> MKKLILLTLIIASFDIYAIDFVYRVDPNPPDVIFR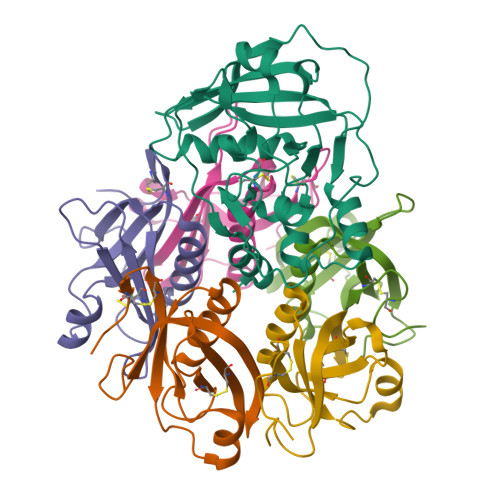DGFSLLGYNRDLQQLISGRSCAGGSSDSRYIVTTSDINKTYAIARAYYSHSKFKGNLYRYKIRADNNFYSLTPSVNYLESQGGHFNAYEKSMIRLQSEYVSTLSILPENIQKAVALVYDSSTGQIKDGTSTINTDYVSISSVSNPGVIPFLPEPQANTQQRIDAFGSLISSCFSIYSVCQTHRGQKTEVYKMPFYDARPVIQFIISGN;>[5x]EWTGDSSINYYSDEVISDFHVGQFNRSAYFCIKTVKKSGEGTPIIACALSHDSKWIPSFNIMLEQARNFYITGHSIRVYVQPNVWSNKSFIEALSSNALVGLSSCSTSECFGPVKP2,2'-[(4-chlorobenzene-1,2-diyl)bis(oxy)]bis(5-nitrobenzonitrile) | C20 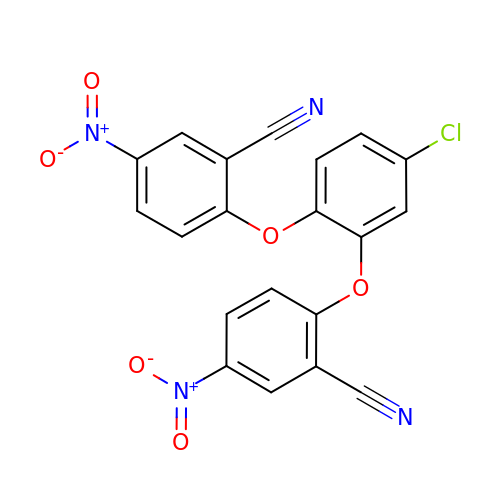H9 Cl N4 O6 | FXXUXJLPGCBXLY-UHFFFAOYSA-N>MSLDVSAYP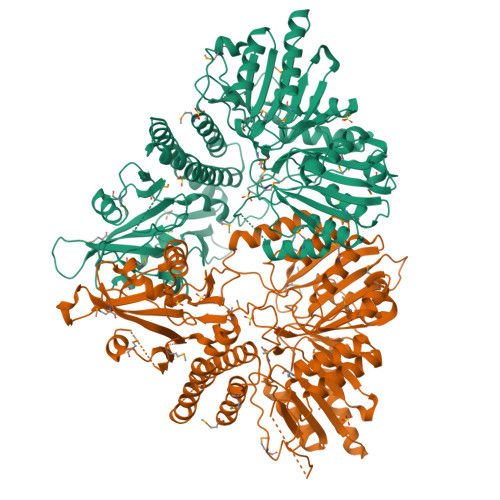FFRRDMSWLSFNERVLMEAADRTLPVYDRIKFLSIFSSNLEEFYTVRVAYHQAVLQKRRDRSEAEEDSDADAHILQAIRETVIRQDELYYRIFYDQILPTLEEHGIRLRTHAPTHPDHKAYLRRFFHEEIFPLLYPMLLLPSKVRTFIRSGRVYLAVRLKEKETDEAYSYALLNVPTDGLPRFVELPRLQTDTFYYYSFLEDIIKEHLDVVFPGYEVMDSYSIKVSRDADLLLDAQRPEDLPGEIRKKVKTRKLGAPTRFMYDGRMPDEVLRYICSSCDIDPEEAIRSGNYVNLQDLAMLPNPFAPRLETLTPEPLLSKHLEQAPSLMEGIRRKDYLIHVPYYTYDYVVRLLMEAAISPDVSEIRLTQYRVAENSSIISALEAAAQSGKKVSVFVELKARFDEENNLRLSERMRRSGIRIVYSMPGLKVHAKTALILYHTPAGERPQGIALLSTGNFNETTARIYSDTTLMTANTDIVHDVYRLFRILDGDPEPARFSRLLVARYNMGEAITNLIEREIENVKRGKRGYMLLKMNGLQDKNVITQLYRASEAGVEIDLIVRGICCLVPDMPQSRNIRVTRLVDMYLEHSRIWCFHNGGKEEVFISSADWMKRNLYNRIETACPVLDPTLRREIIDILEIQLRDNIKACRIDSSLNNIYKHNSDEKPVRAQAAIYRYLKGKEETTPAAKEGHHHHHH[2x]>[3x]MAHHHHHHDDDDKIRTLPGEGTQVHPRAPLLQILKVAGAQEEVFTLKEVMHYLGQ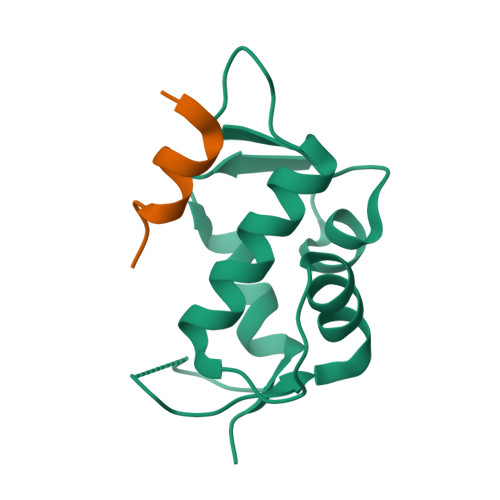YIMMKQLYDKQRQHIVHCHDDPLGELLEVGSFSVKNPSPVYEMLKRNLVILNNSDAAKNLSVGKDSNESPSEDPGQVSSGSINSA;>[3x]SQETFSDLWKLLPEN>GSHMVVKFTDSQIQHLMEYGDNDWSEAEFEDAAARDKEFSSQFSKLKSANDKGLKDVIANPRNDLTDLENKIREKLAARGFIEVHTPIFVSKSALAKMTITEDHPLFKQVFWIDDKRALRPMHAMNLYKVMRELRDHTKGPVKIFEIGSCFRKESKSSTHLEEFTMLNLVEMGPDGDPMEHLKMYIGDIMDAVGVEYTTSREESDVYVETLDVEINGTEVASGAVGPHKLDPAHDVHEPWAGIGFGLERLLMLKNGKSNARKTGKSITYLNGYKLD[10x]

Site-specific incorporation of non-canonical amino acids into proteins in response to specified (e.g., UAG) codons has been achieved by pairs of an engineered aminoacyl-tRNA synthetase (aaRS) and tRNA, including the pairs of pyrrolysyl-tRNA synthetase (PylRS) and tRNAPyl (CUA). The PylSc-type PylRS from the methanogenic archaeon ISO4-G1 (ISO4-G1 PylRS) is highly similar to MaPylRS with 64% sequence identity, while ISO4-G1 PylRS and MaPylRS both share around 38% sequence identity with M. mazei PylRSc. The genome of the methanogenic archaeon ISO4-G1 encodes an ISO4-G1 PylRS protein consisting of 273 amino acids, which is quite similar to MaPylRS. The following residues Asn60-Asp273 constitute the catalytic domain, with the characteristic topology of the class-II aaRSs: an extended six-strand, anti-parallel β-sheet (β3, β4, β5, β6, β7, β8) surrounded by α-helices.

The crystallization of the ISO4-G1 PylRS protein was successful when using PEG3350 as the precipitant, and the crystal structure of the ISO4-G1 PylRS apo form has been determined at 2.78-Å resolution. The asymmetric unit contains ten molecules of PylRS (five PylRS dimers, A/B, C/G, D/F, E/H, J/I). In the ISO4-G1 PylRS structure, the residues from Met1 to Pro58 contain two α-helices (α1 and α2). The structures of the ordering loop (residues Ile97-Gln106) and the motif-2 loop (residues Lys150-Glu159) are quite similar in the ten PylRS molecules, while the β5-β6 hairpin (residues Thr195-Ile212) adopts open and closed conformations. Tyr204, at the tip of the β5-β6 hairpin in ISO4-G1 PylRS molecules A, C, E, F, and J, is located far from the amino acid binding pocket (the open conformation), while in ISO4-G1 PylRS molecules B, D, G, H, and I, Tyr204 is located inside the amino acid binding pocket (the closed conformation). Interestingly, the ISO4-G1 PylRS structure revealed that the His225 residue (corresponding to His227 in MaPylRS) undergoes drastic conformational changes in accordance with the location of the Tyr204 residue (corresponding to Tyr206 in MaPylRS) in the β5-β6 hairpin. On the one hand, when Tyr204 is far from the amino acid binding pocket (the open conformation), a π–π stacking interaction is observed between the imidazole ring of His225 and the indole ring of Trp237. On the other hand, when Tyr204 is located inside the amino acid binding pocket (the closed conformation), the imidazole ring of His225 shifts and is stabilized by a π–π stacking interaction with the aromatic ring of Tyr204. In ISO4-G1 PylRS, the Met128 side-chain protrudes into the amino acid binding pocket, which would reduce the pocket size as compared with that of MmPylRSc. Based on the crystal structure of ISO4-G1 PylRS, the β5–β6 hairpin may exist in a dynamic open-closed equilibrium, and the location and conformational change of the His225 residue appear to be important for the catalytic activity.> MESLTLQPIARVDGTINLPGSKSVSNRALLLAALAHGKTVLTNLLDSDDVRHMLNALTALGVSYTLSADRTRCEIIGNGGPLHAEGALELFLGNAATAMRPLAAALCLGSNDIVLTGEPRMKERPIGHLVDALRLGGAKITYLEQENYPPLRLQGGFTGGNVDVDGSVSSQFLTALLMTAPLAPEDTVIRIKGDLVSKPYIDITLNLMKTFGVEIENQHYQQFVVKGGQSYQSPGTYLVEGDASSASYFLAAAAIKGGTVKVTGIGRNSMQ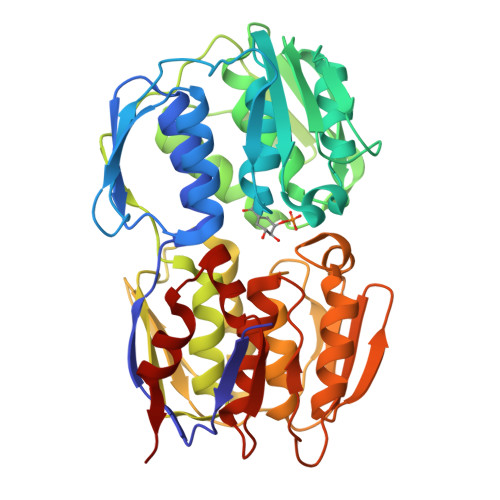GDIRFADVLEKMGATICWGDDYISCTRGELNAIDMDMNHIPDAAMTIATAALFAKGTTTLRNIYNWRVKETDRLFAMATELRKVGAEVEEGHDYIRITPPEKLNFAEIATYNDHRMAMCFSLVALSDTPVTILDPKCTAKTFPDYFEQLARISQAA> MVILGVGYFLLGLILLYYGSDWFVLGSERIARHFNVSNFVIGATVMAIGTSLPEILTSAYASYMHAPGISIGNAIGSCICNIGLVLGLSAIISPIIVDKNLQKNILVYLLFVIFAAVIGIDGFSWIDGVVLLILFIIYLRWTVKNGSAEIEENNDKNNPSVVF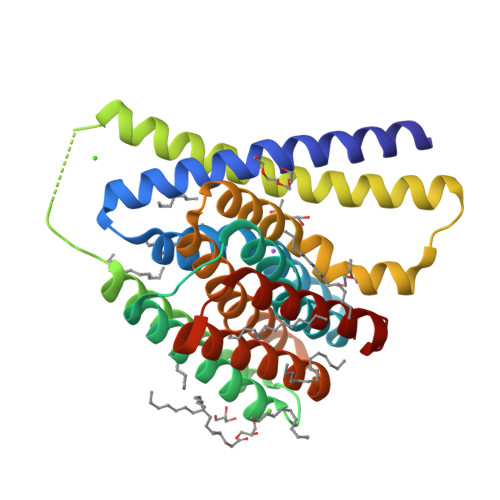SLVLLIIGLIGVLVGAELFVDGAKKIALALDISDKVIGFTLVAFGTSLPELMVSLAAAKRNLGGMVLGNVIGSNIADIGGALAVGSLFMHLPAENVQMAVLVIMSLLLYLFAKYSKIGRWQGILFLALYIIAIASLRMGGG> DAAKLRALLWTPPP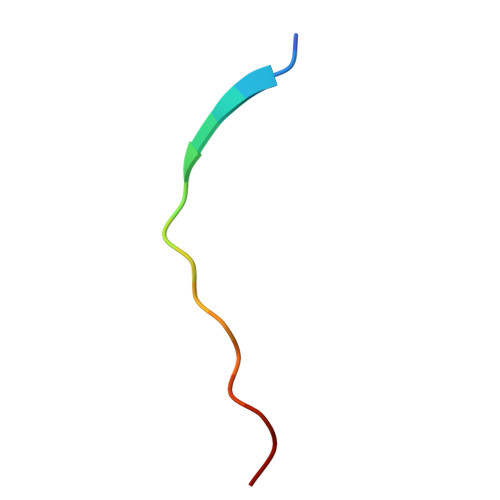TP(2R,3R)-N-[(1-{(3S,3aR,6S,6aR)-6-[4-({[(2R,3R)-2,3-dihydroxy-4-oxo-4-{[(2R,3R,4R,5R,6R)-3,4,5-trihydroxy-6-(hydroxymethyl)tetrahydro-2H-pyran-2-yl]amino}butanoyl]amino}methyl)-1H-1,2,3-triazol-1-yl]hexahydrofuro[3,2-b]furan-3-yl}-1H-1,2,3-triazol-4-yl)methyl]-2,3-dihydroxy-N'-[(2R,3R,4S,5R,6R)-3,4,5-trihydroxy-6-(hydroxymethyl)tetrahydro-2H-pyran-2-yl]butanediamide (non-preferred name) | C32 H48 N10 O20 | 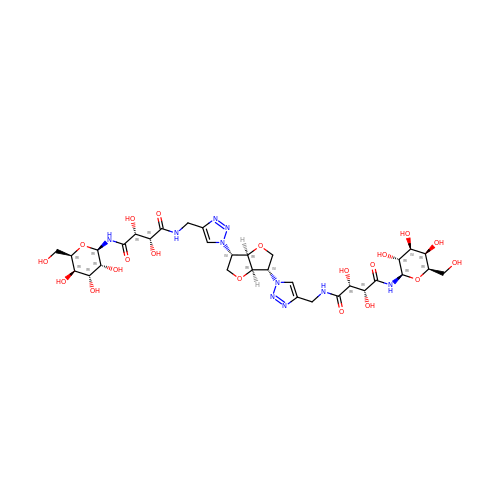JJYDUQGILJLGLW-XRTDXAHQSA-N> GLELLIAQTILQGFDAQYGRFLEVTSGAQQRFEQADWHAVQQAMKNRIHLYDHHVGLVVEQLRCITNGQSTDAEFLLRVKEHYTRLLPDYPRFEIAESFFNSVYCRLFDHRSLTPERLFIFSSQPERRFRTIPRPLAKDFHPDHGWESLLMRVISDLPLRLHWQNKSRDIHYIIRHLTETLGPENLSKSHLQVANELFYRNKAAWLVGKLITPSGTLPFLLPIHQTDDGELFIDTCLTTTAEASIVFGFARSY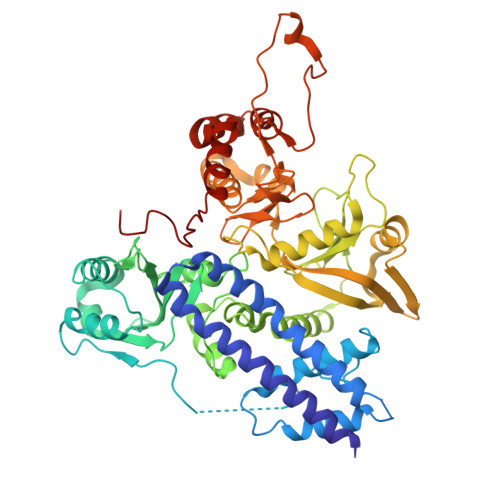FMVYAPLPAALVEWLREILPGKTTAELYMAIGCQKHAKTESYREYLVYLQGCNEQFIEAPGIRGMVMLVFTLPGFDRVFKVIKDKFAPQKEMSAAHVRACYQLVKEHDRVGRMADTQEFENFVLEKRHISPALMELLLQEAAEKITDLGEQIVIRHLYIERRMVPLNIWLEQVEGQQLRDAIEEYGNAIRQLAAANIFPGDMLFKNFGVTRHGRVVFYDYAEICYMTEVNFRDIPPPRYPEDELASEPWYSVSPGDVFPEEFRHWLCADPRIGPLFEEMHADLFRADYWRALQNRIREGHVEDVYAYRRRQRFSV>[5x]STTEVVMENVT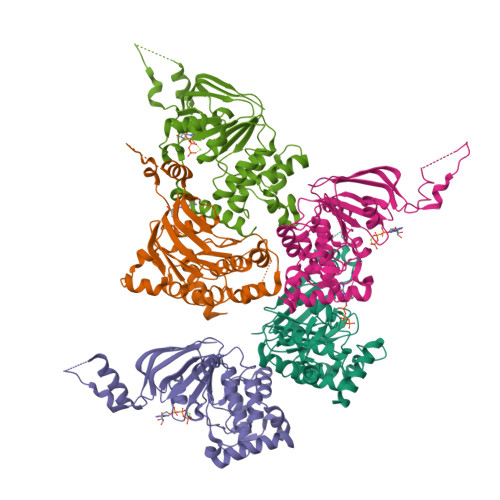AFWEEGFGELFEKAKQNNNNRKTSNGDDSLSFSNFSLLGTPVLKDINFKIERGQLLAVAGSTGAGKTSLLMMIMGELEPSEGKIKHSGRISFCSQFSWIMPGTIKENIIAGVSYDEYRYRSVIKACQLEEDISKFAEKDNIVLGEGGITLSGGQRARISLARAVYKDADLYLLDSPFGYLDVLTEKEIFESCVCKLMANKTRILVTSKMEHLKKADKILILHEGSSYFYGTFSELQNLQPDFSSKLMGCDSFDQFSAERRNSILTETLRRFSLEGDAPVS>[7x]XGEIAQALKEIAKALK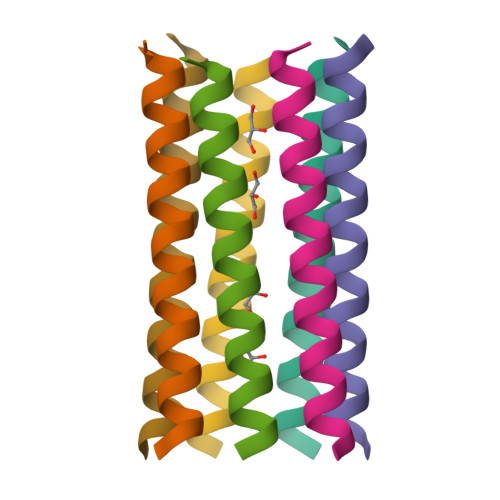EIAWALKEIAQALKG> GSETHRRVRLL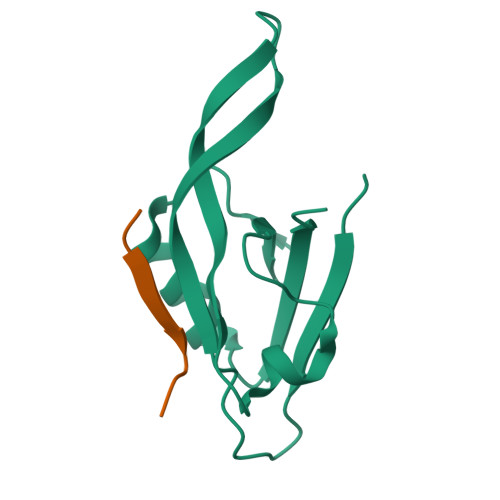KHGSDKPLGFYIRDGTSVRVTASGLEKQPGIFISRLVPGGLAESTGLLAVNDEVIEVNGIEVAGKTLDQVTDMMVANSSNLIITVKPANQR;> YPKHREMAVDCP>GAMATSDTQKAMAMLIATFHKYSGKEGDKLTLSKGELKELLSAELGDIFGKTTDKAALDKIFKDLDANADGSVDFQEYITLIACITMLCNEFFT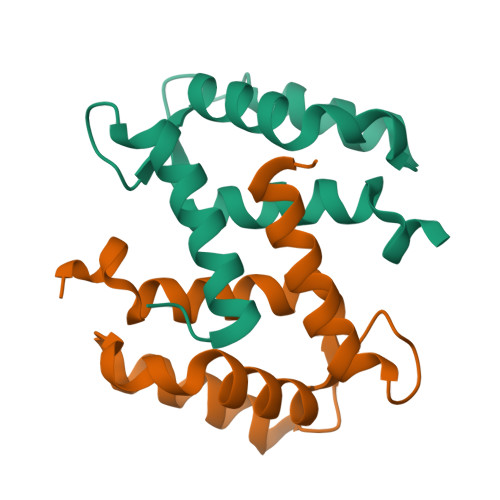GKK[4x]> GPGSMRLGRIASPDGVAFAS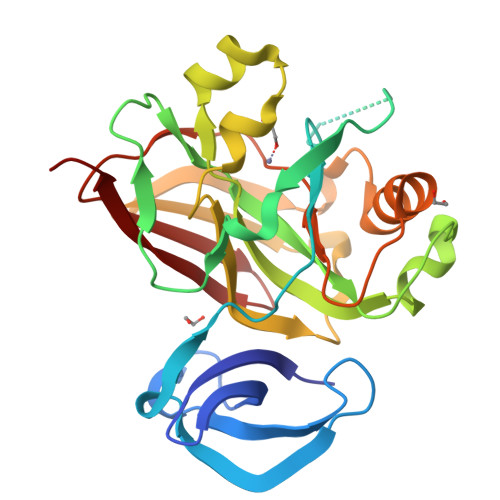IEGELDNPGAMTAREIAEHPFGTPNFTGRSWPLADVRLLAPILASKVVCVGKNYTDHIAEMGGQTGPTPADPVIFLKPNTAIVGPNVPIRLPANASPVHFEGELAIVIGRPCKDVSAAQAVDNILGYTIGNDVSARDQQKSDGQWTRAKGHDTFCPVGPWIVTDVDPADLELRTEVNGAVKQHARTSLMIHDVGAIVEWISAVMTLLPGDLILTGTPAGVGPIEDGDTVSITIEGIGTLTNPVVRKGK> MSSLSRELVFLILQFLDEEKFKETVHKLEQESGFFFNMKYFEEKVHAGEWDEVEKYLSGFTKVDDNRYSMKIFFEIRKQKYLEALDRHDRAKAVDILVKDLKVFSTFNEELYKEITQLLTLENFRENEQLSKYGDTKSARSIMLIELKKLIEANPLFREKLVFPTLKASRLRTLINQSLNWQHQLCKNPRPNPDIKTL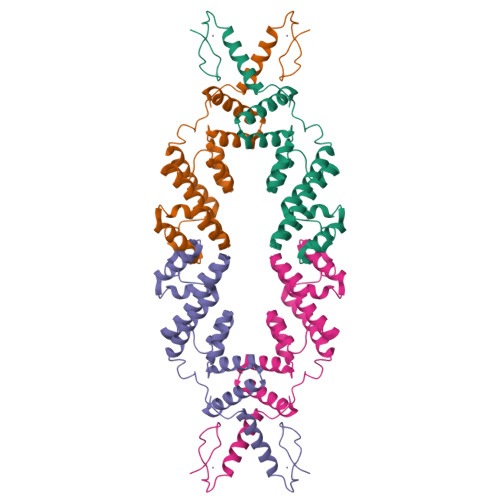FTDHTCTPPNG>PMFIVNTNVPRASVPDGFLSELTQQLAQATGKPPQYIAVHVVPDQLMAFGGSSEPCALCSLHSIGKIGGAQNR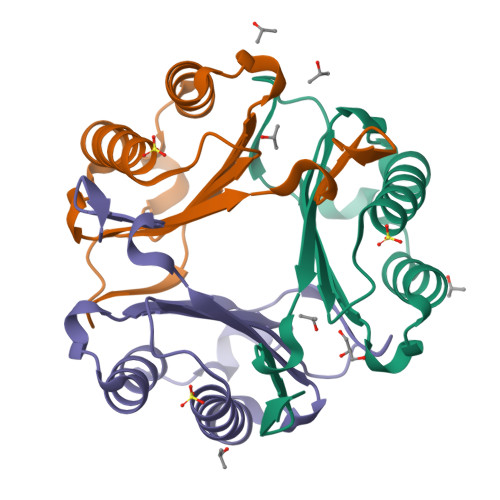SYSKLLCGLLAERLRISPDRVYINYYDMNAANVGWANSTFA[3x]>[2x]GSHMSLSGKIAAVTGAAQGIGKAIALRLAKDGADVILLDVKQDTLAETAKEVEALGRRAVALTADISNRDQFRSTLADAAKTLGGLDIMVNNAGICQVKPILDIEPAEIEKIFSINVQGVLWGMQAAATLFKEKGTKGKIINACSIAGHEGYPLLGA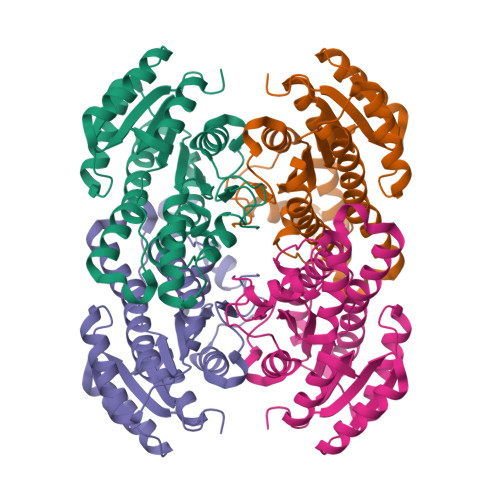YSATKFAVRALTQSAAKELASSGITVNSYCPGIVGTDMWVTIDKRMAEITGTEIGATYKKYVEGIALGRVETADDVAGFVAYLSSSDADYMTGQSVLIDGGLVFR>[3x]ACDYTCGSNCYSSSDVSTAQAAGYKLHEDGETVGSNSYPH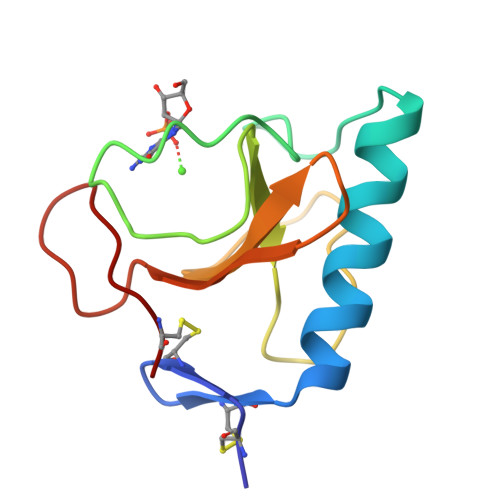EFRNWQGFDFSVSSPYYEWPILSSGDVYSGGSPGADRVVFNENNQLAGVITHTGASGNNFVECT> GLEDCDFGWSPYDQHCYQAFNEQKTWDEAEKFCRAQENGAHLASIESNGEADFVSWLISQKDELADEDYVWIGLRAQNKEQQCSSEWSDGSSVSYENLIDLHTKKCGALEKLTGFRKW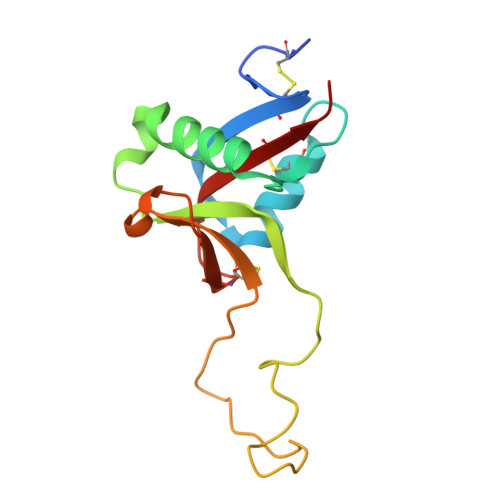VNYYCEQMHAFVCKLLPY>[2x]SMGEAICSALPTIPYHKLADLRYLSRGASGTVSSARHADWRVQVAVKHLHIHTPLLDSERKDVLREAEILHKARFSYILPILGICNEPEFLGIVTEYMPNGSLNELLHRKTEYPDVAWPLRFRILHEIALGVNYLHNMTPPLLHHDLKTQNILLDNEFHVKIADFGLSKWRMMSLSQSRSSKSAPEGGTIIYMPPENYEPGQKSRASIKHDIYSYAVITWE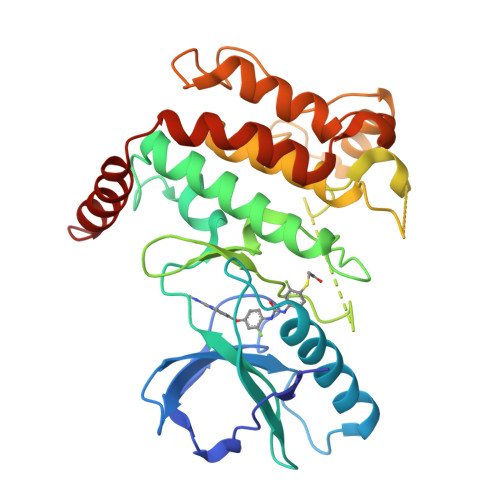VLSRKQPFEDVTNPLQIMYSVSQGHRPVINEESLPYDIPHRARMISLIESGWAQNPDERPSFLKCLIELEPVLRTFEEITFLEAVIQLKKTKLQSV> IQCDELVHAESKSITCKSASGNEKECSVTGRALLPAVNPGQEACLHFSMPGSPDSKCLKIKVKSINLRCKQASSYYVPEAKARCTSVRRCRWAGDCQSGCPTYFSSNSFSDDWANRMDRAGLGMSGCSDGCGGAACGCFNAAPSCIFWRKWVENPSNRVWKVSPCASWVLAAIIELTLPSGEVKTLEPVTGQATQMFKGVAITYLGSSIEIVGMTRLCEMKEMGTGIMALAPCNDPGHAIMGNVGEIQCSSIESAKHIRSDGCIWNADLVGIELRVDDAVCFSKLTSVEAVANFSKIPAIISGVRFDQGNHGESRIYGSPLDITKVSGEFSVSFRGMRLKLSEISASCTGEITNVSGCYS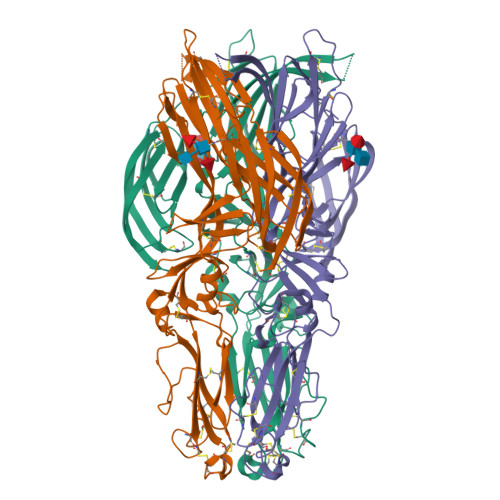CMTGASVSIKLHSSKNTTGHLKCDSDETAFSVMEGTHTYRPHMSFDKAVVDEECVLNCGGHSSKLLLKGSLVFM>[2x]MKELFQKIWQNELQFLNFDAKFQDKSKLDTAECAIILSVNKDNYERYFLLKEFQELCKKIDLRVDIFSMQNAQICILNLFKSGFISKQDLLKALKILEKISKNTEIFDFILQEKVQSIDQKALFQNDF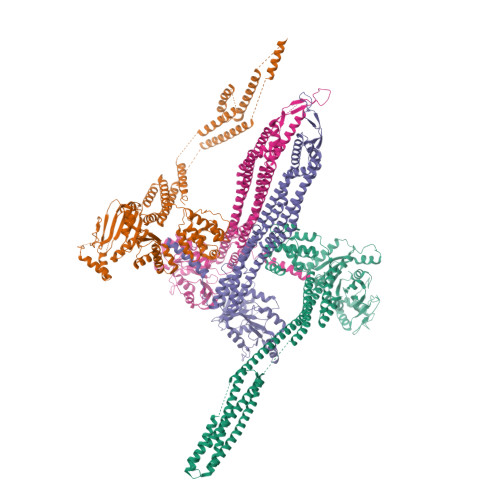KELNTINLELQKLSFDENLKSRLQKTLEKFQNLEFNIAITGVMNAGKSSLLNALLKEDFLGVSNIPETANLTVLSYGKSEEAKIYFWDKKEWQNILESSHFNADLKEFIDKLDKSVNIEDFIKDKPLIQNIALCELKNFSSAKNKISALIKKIEIKSHLEFLKNNISIVDTPGLDDVVVQREIVTNEYLRESDFLIHLMNASQSLTQKDADFLVHCLLNSRLSKFLIVLTKADLLSKKDLEEVIVYTKESLKSRLVDLDENLVEKIDFLCVSAKMASDFYKGLASKESLQKSGMQEFENYLFNELYAGEKSKIALRAYKKELHLELKNILSEYEMQNRLIKENKQGVSEENQKLLLELQKQNTLLKEAQDEISNSIAKLKNIDSGIDNLVLLLAKKLKERLIDEFKYLKNNAQKLNLSRILNIVDITTKDGINDILREIKFENIKKIEELKTNLSLKYDFLKDDFDNGFEGFKDGISKNIDSIFQSEKFALLRLKIEKLSNLKSDLYELETNLDTVIFDTFKEFKMSEILNSLNINGAFFEFLNDKLKHYEKNQKSKLESLEKVLQSLKNQDANILNSFEENLEKIEKLKQLEMGLLNADKLHH;>GSHMQINLLNDFIKAYENTYSVSFDDSFKGRIQELCKELNEPFMHASYALENELKELVFSLDKNVNIAIIGQFSSGKSSLLNLILGRDCLPTGVVPVTFKPTFLRYAKEYFLRVEFEDGSDIITNIEKLAFYTDQRNEVKQAKSLHIFAPIPLLEKITLVDTPGLNANENDTLTTLDELKNIHGAIWLSLIDNAGKKSEEDAIKANLELLGENSICVLNQKDKLSAEELDNVLNYAKSVFLKYFNELIAISCKEAKDEQSYEKSNFQSLLDFLTQLDTTVLKEKFVKRKILNLCEILEDENQLFVGIFDRLLNQFQSYEKHLLLAYENFLKEIEILNHQILEQLKSISERISSEIFASVKEKDAYFYKESKGFLKKDLYTRYDYKAPYISSDDAFLAMFYNSDVMSKEFKKIKNELYKSFEEIKMKLKDFINILEREILLFKAEFSNIQKDHIFQSDKNFSELRAFCNASDEYFLKDFKELLFKSILELDLFFEKLNLKAFTNYENATKLSLAFFSRKINESRVLYELDSSEFVLFYPKKSEIYERVLNELNVYEFETLLINKPILTKIAKNFLEQSQNLIQEKNKFLDLKKAELQKRRAQILNVRESIKEDHH[2x]> MDLADRFAELARRYDARLGVYVPATGTTAAIEYRADERFAFCSTFKAPLVAAVLHQNPLTHLDKLITYTSDDIRSISPVAQQHVQTGMTIGQLCDAAIRYSDGTAANLLLADLGGPGGGTAAFTGYLRSLGDTVSRLDAEEPELNRDPPGDERDTTTPHAIALVLQQLVLGNALPPDKRALLTDWMARNTTGAKRIRAGFPADWKVIDKTGTGDYGRANDIAVVWSPTGVPYVVAVMSDRAGGGYDAEPREA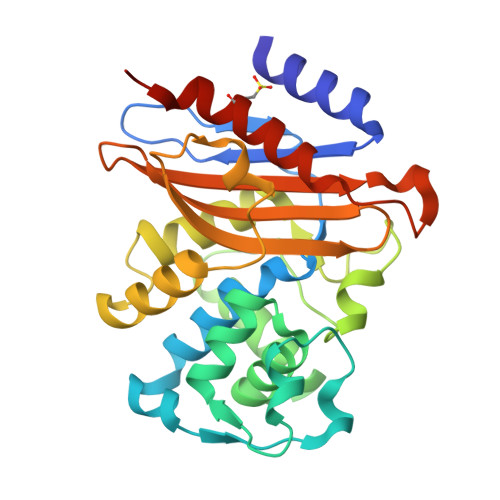LLAEAATCVAGVLALEHHHHHH>[2x]GAMGSGMAMDTFITRNFQTTIIQKAKNTMAEFSEDPELQPAMLFNTCVHLEVCYVISDMNFL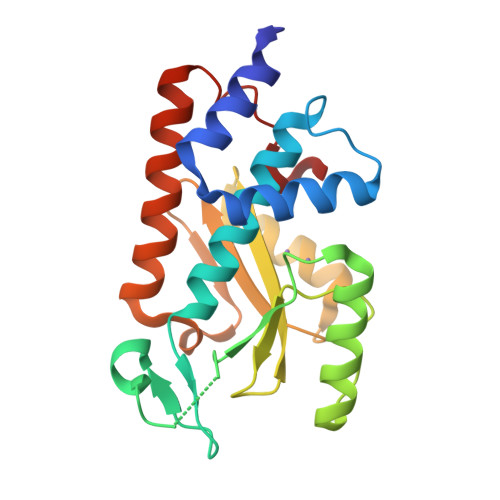DEEGKSYTALEGQGKEQNLRPQYEVIEGMPRTIAWMVQRSLAQEHGIETPKYLADLFDYKTKRFIEVGITKGLADDYFWKKKEKLGNSMELMIFSYNQDYSLSNESSLDEEGKGRVLSRLTELQAELSLKNLWQVLIGEEDVE> EFAITSCPNNETVWETPIGVKYTLCPGS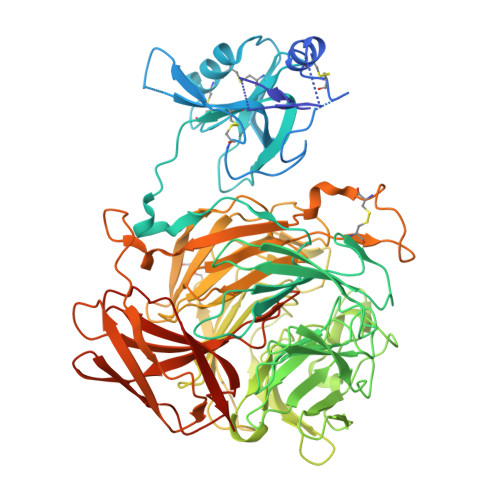DYQNGGASLQTVRDIQSSLECAKICDSDARCNRAVYDNVNKACDVKNSTNPMQWAADDRFETIRLTNDLPEGAFISTCSFNETSYRVPETNAEYRICPDTDYTGVNAKVVEGVTTIQACAELCSNTQDCRKSVFDHINNACAIKAAEPATSIFWVQDKQFSTIRLPENIDPAVKGKWGDLIRLPVIPVAAYIVPSYPEPSRLLFFSSWSNDAFSGASGMTQFGDYDFATGAISQRTVTNTHHDMFCPGISQLEDGRILIQGGSDADTVSIYDPATNEFTRGPNMTLARGYQTSCTLSNGKVFTIGGAFSGERVGKNGEVYDPVANAWTYLPGADFRPMLTNDHEGIWREDNHAWLFGWKNGSIFQAGPSKDQHWYGIQGNGTVAKAATRDDDDAMCGVWVMYDAVAGKIFSAGGSPDYTDSPATQRAHITTIGEPNTPAEVERVADMGFPRGFANAVVLPDGQVLVTGGQRMSLVFTNTDGILVAELFNPETREWKQMAPMAVPRNYHSVSILLPDATVFSGGGGMCWVQNVGDSTAGCDKTVDHSDGEIFEPPYLFNEDGSRAARPVISAISADPIKAGATLTFTVEGVEGQGTAALIRLGSVTHSVNSDQRRVPLNVTVSGNEYSATLPDDYGILLPGYYYLFVSTPQGTPSIAKTVHVILGLEQKLISEEDLNSAVDHHHHHH>[2x]MNNRNHDVLSRMISEKAALHGLLNCLIKEFAIPEGYLRYEWPDEMKGIPPGAYFDGADWKGIPMMIGLPDQLQLFVMVDRRDTFGSQHYLSDVYLRQAQGDWQCPDFEPLVARLLAACEHIAGRKNPELYEQILQSQRLVSAIVSHNGRQRADAPLQHYLQSEQGLWFGHPSHPAPKARLWPAHLGQEQWAPEFQARAALHQFEVPVDGLHIGANGLTPQQVLDGFADQQPASPGHAIICMHPVQAQLFMQDARVQQLLRD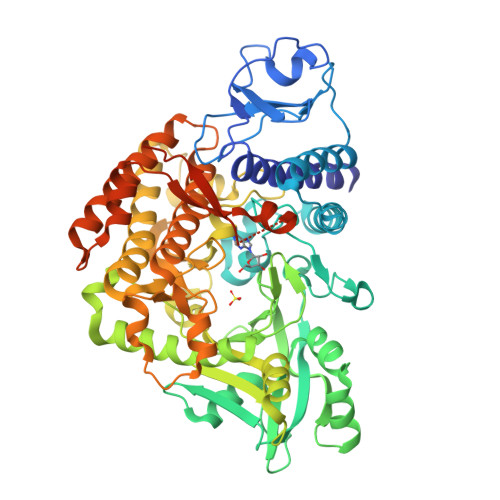NVIRDLGQSGRVASPTASIRTWFIDDHDYFIKGSLNVRITNCVRKNAWYELESTVLIDRLFRQLLDQHADTLGGLVAAAEPGVVSWSPAAAGELDSHWFREQTGGILRENFCRRTGAERSIMAGTLFARGVDLQPMIQTFLRTHYGEALDDNALLYWFDDYQTRLLRPVLSLFFNHGVVMEPHLQNSVLVHQQGRPQQVLLRDFEGVKLTDDLGIRYIDDDIHPRVRQSLLYSREQGWNRIMYCLFINHLSETILALSQGRPQLAPLMWRRVQQQLRAIQGELKQPSPELDALIAGHPVACKTNLKVRLAAEADRQASYVRLPSPWGHAVQHGSEVQHDERRHGDVRHEEARHGEVQHG3-[[6-(cyclohexylmethoxy)-7~{H}-purin-2-yl]amino]-~{N}-[3-(dimethylamino)propyl]benzenesulfonamide 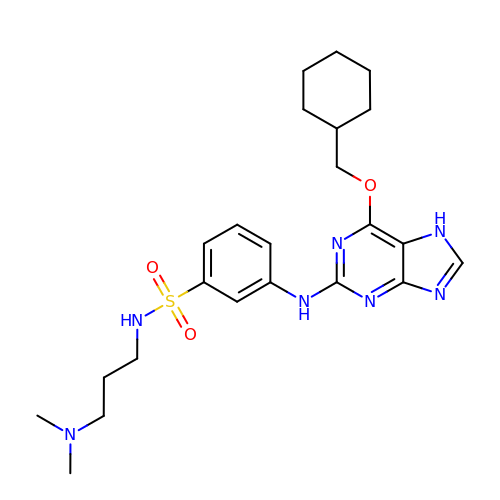| C23 H33 N7 O3 S | PEEXIAQHZDNIBT-UHFFFAOYSA-N>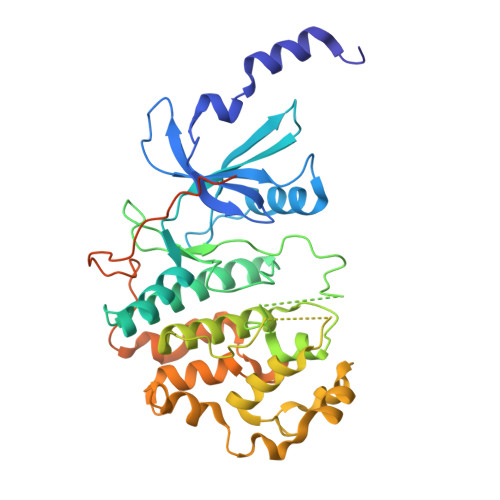 DKMDYDFKVKLSSERERVEDLFEYEGCKVGRGTYGHVYKAKRKDGKDDKDYALKQIEGTGISMSACREIALLRELKHPNVISLQKVFLSHADRKVWLLFDYAEHDLWHIIKFHRASKANKKPVQLPRGMVKSLLYQILDGIHYLHANWVLHRDLKPANILVMGEGPERGRVKIADMGFARLFNSPLKPLADLDPVVVTFWYRAPELLLGARHYTKAIDIWAIGCIFAELLTSEPIFHCRQEDIKTSNPYHHDQLDRIFNVMGFPADKDWEDIKKMPEHSTLMKDFRRNTYTNCSLIKYMEKHKVKPDSKAFHLLQKLLTMDPIKRITSEQAMQDPYFLEDPLPTSDVFAGCQIPYPKREFLTEEEPDDKGDKKNQQQQQGNNHTNGTGHPGNQDSSHTQGPPLKK> MKICLIDETGAGDGALSVLAARWGLEHDEDNLMALVLTPEHLELRKRDEPKLGGIFVDFVGGAMAHRRKFGGGRGEAVAKAVGIKGDYLPDVVDATAGLGRDAFVLASVGCRVRMLERNPVVAALLDDGLARGYADAEIGGWLQERLQLIHASSLTALTDITPRPQVVYLDPMFPHKQKSALVKKEMRVFQSLVGPDLDADGLLEPARLLATKRVVVKRPDYAPPLANVATPNAVVTKGHRFDIYAGT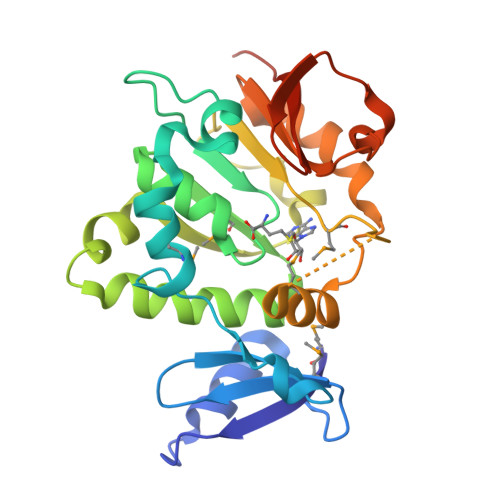PVLEHHHHHH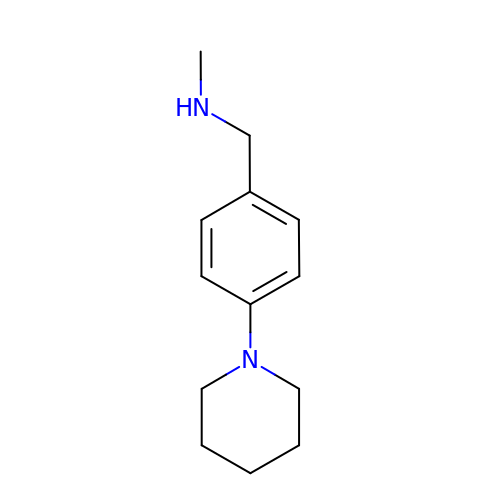~{N}-methyl-1-(4-piperidin-1-ylphenyl)methanamine | C13 H20 N2 | ABHBNGLDUNAXSR-UHFFFAOYSA-N>QNVSLQPPPQQLIVQNKTIDLPAVYQLNGGEEANPHAVKVLKELLSGKQSSKKGMLISIGEKGDKSVRKYSRQIPDHKEGYYLSVNEKEIVLAGNDERGTYYALQTFAQLLKDGKLPEVEIKDYPSVRYRGVVEGFYGTPWSHQARLSQLKFYGKNKMNTYIYGPKDDPYHSAPNWRLPYPDKEAAQLQELVAVANENEVDFVWAIHPGQDIKWNKEDRDLLLAKFEKMYQLGVRSFAVFFDDISGEGTNPQKQAELLNYIDEKFAQVKPDINQLVMCPTEYNKSWSNPNGNYLTTLGDKLNPSIQIMWTGDRVISDITRDGISWINERIKRPAYIWWNFPVSDYVRDHLLLGPVYGNDTTIAKEMSGFVTNPMEHAESSKIAIYSVASYAWNPAKYDTWQTWKDAIRTILPSAAEELECFAMHNSDLGPNGHGYRREESMDIQPAAERFLKAFKEGKNYDKADFETLQYTFERMKESADILLMNTENKPLIVEITPWVHQFKLTAEMGEEVLKMVEGRNESYFLRKYNHVKALQQQMFYIDQTSNQNPYQPGVKTATRVIKPLIDRTFATVVKFFNQKFNAHLDATTDYMPHKMISNVEQIKNLPLQVKANRVLISPANEVVKWAAGNSVEIELDAIYPGENIQINFGKDAPCTWGRLEISTDGKEWKTVDLKQKESRLSAGLQKAPVKFVRFTNVSDEEQQVYLRQFVLTIEKK[2x]

The enzyme responsible for removing O-GlcNAc from proteins is O-GlcNAcase (OGA),23 which is a member of glycoside hydrolase family 84 (GH84) of the CAZy classification system. Inhibitors of O-GlcNAc hydrolase (OGA), the enzyme that removes O-GlcNAc from proteins, lead to increased O-GlcNAc levels in cells and are seeing widespread adoption in the field as a research tool used in cells and in vivo. Structures of bacterial OGA homologues, in which the active site residues are completely conserved with hOGA,34,35 show a discretely sized pocket having a volume that nicely accommodates the propyl substituent of 15d. Structural data of inhibitors in complex with an hOGA homologue reveals the basis for variation in binding among these compounds.

A butyl chain, however, leads to a greater than 100-fold loss of potency (15e, Ki = 350 nM). To assess the structural basis for this stepped decrease in potency observed on going to the 2′-aminobutylthiazoline 15e, we determined the structure of Bacteroides thetaiotaomicron, a bacterial homolog (BtGH84) of hOGA, in complex with the parent 2′-aminothiazoline 11a, the tighter binding 2′-aminopropylenethiazoline 11b, and the butyl derivative 15e, which shows greatly diminished binding. In all three structures, the respective inhibitor binds in the active site in a conserved mode with an invariant hydrogen bond pattern for the aminothiazoline moiety. Even a small further extension of the alkyl chain, as in the butyl derivative 15e, leads to steric clashes with multiple residues in the cavity, driving the side chain of C278 to adopt a different orientation. Furthermore, we observe the polypeptide main chain surrounding C278 is shifted away from the inhibitor. Thus, the size of the pocket disfavors substituents longer than three carbon units in chain length, and those inhibitors having such larger groups induce unfavorable conformational changes within the active site. We also noted that the selectivity ratio for hOGA increases as the 2′-aminoalkyl chain length increases to the three-carbon propyl (15d) and propylene (11b) derivatives, but this trend reverses once the chain length increases further, as seen for the 2′-aminobutyl analogue (15e). Since the active site pocket for hHexB is more constrained in the vicinity of the acetamido group, these observations are consistent with structural observations of both bacterial hOGA homologues and hHexB. This suggests that once the 2′-substituent passes the volume that can be accommodated in the active site of hOGA, increases in bulk are even slightly more deleterious for hOGA as compared to hHexB.>[2x]MDTVNNYRVLEHKAAGHDGTLTDGDGLLIFKPAFPQELEFYKAIQVRDVSRRKSSADGDAPLCSWMPTYLGVLNEGAKIEQSGDAALLKIDERLSDSTDNLDSIPVKSEKSKQYLVLENLLYGFSKPNILDIKLGKTLYDSKASLEKRERMKRVSETTTSGSLGFRICGMKIQKNPSVLNQLSLEYYEEEADSDYIFINKLYGRSRTDQNVSDAIELYFNNPHLSDARKHQLKKTFLKRLQLFYNTML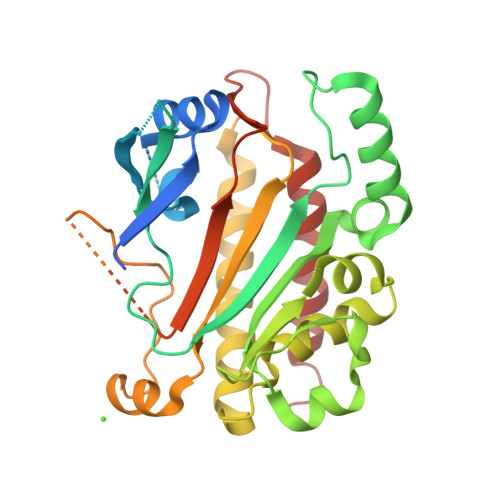EEEVRMISSSLLFIYEGDPERWELLNDVDKLMRDDFIDDDDDDDDNDDDDDDDAEGSSEGPKDKKTTGSLSSMSLIDFAHSEITPGKGYDENVIEGVETLLDIFMKFLEHHHHHH>[6x]GSLRGTTQKVNRIRE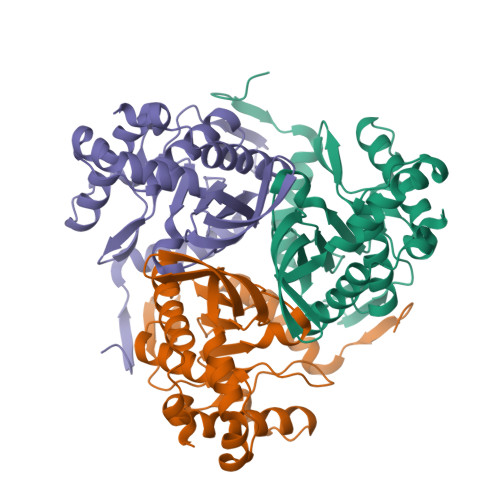ITAMKTVEALQISAQLTQLHEVDMTRVAELRKKNKPAFIEKHGVNLTYLPFFVKAVVEALVSHPNVNASFNAKTKEMTYHSSVNLSIAVDTPAGLLTPVIHDAQDLSIPEIAKAIVDLADRSRNNKLKPNDLSGGTFTITNIGSEGALSDTPILVPPQAGILGTGAIVKRPVVITEDGIDSIAIRQMVFLPLTYDHQVVDGADAGRFLTTIKDRLETANFEGDLQL> GDYTAYPWFAGNMERQQTDNLLKSHASGTYLIRERPAEAERFAISIKFNDEVKHIKVVEKDNWIHITEAKKFDSLLELVEYYQCHSLKESFKQLDTTLKYPY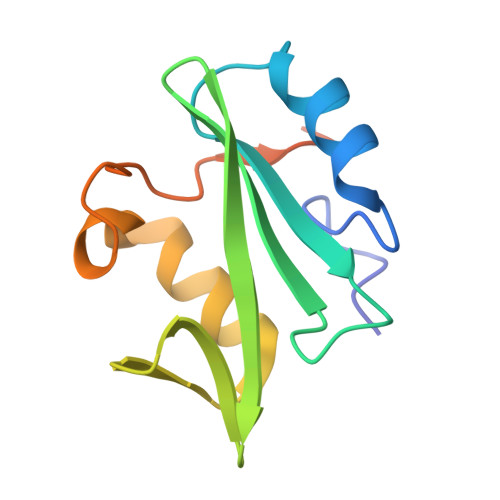KSRERSASRASSRSP>SHMMPLQSLVKALWNVLHEEESEGYPDLTELIAEVESYQQRYPKQNPTNSQKIRHILDEIYEKTPFNNTRRRILWL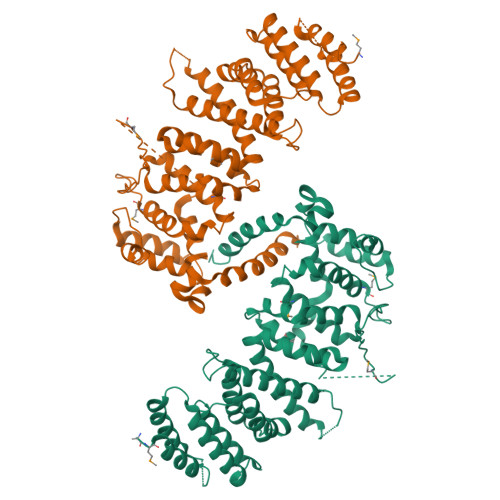AVLKTVIPLLILDRQAVGEWWDQIFFPFLNSPTQLKPVFSDLKSILFYILIFHDEDEWGGDLRRECAEETITRLVDLYVSKAIENLGDVESQEQRNQTIECLVNVLVHYGIQRPKELSSCFCHHFLNPPTRIPILSVMVEVIRRQGPRLYEIPQTGFYDLVLKCAEFDTSPILLSYALSFILMILSHICNSLDDSLYRLFCIYLRFSMIDPTSGFPSSTASGNWEVFHDFMSTYASTTTSQTDSSYNDVHDIVGSSQPDYLESLDYSQLFSILYALYPINFLEFLRDPKLYASKHNFQIRYSFNQELLSTKSDGLLGRHLAHSNFLKYTAETELTDKSRWTRLDSIAVVALCNSLNAV[20x]NsP1 is the membrane anchor for the complex, forming dodecameric pores that associate monotopically with the membrane in the necks of the spherules to gate their entrance. Enzymatically, nsP1 also has a role in addition of cap0 structures to the 5′ end of the positive-sense viral RNAs. NsP1 possesses both N′7 methyltransferase and guanylyltransferase activity and reverses the order of these reactions. Each nsP1 protomer is built around a methyltransferase fold common to SAM-dependent methyltransferases with additional insertions (membrane binding and oligomerisation (MBO) loops 1 and 2) and extensions (ring aperture membrane binding oligomerisation (RAMBO) domain) that contribute to pore formation, oligomerization, and membrane binding.

The GTP pocket in the capping domain of nsP1 is defined by the tip of strand β4, loop β4-αD, and helix αZ, where loops αC-β4 and β4-αD communicate with the adjacent SAM site. The guanosine base fits in a hydrophobic pocket defined by residues D152, Y248, F241 (β10-11 lid), Y154 (β4-αD loop), and F178 (β5). Base stacking occurs in between D152 and Y248, where the latter residue changes rotamer relative to the SAM-bound and apo structures to become planar with the guanosine. E250 of strand β11 forms H-bonds to the N1 and N2 of the guanosine base, and the carboxylate group of residue D152 (β4-αD loop) maintains a network of H-bonds with GTP-O6 and N7 through an intermediate water molecule. However, relative to other N7 MTases, the GTP pocket is deeper in nsP1, and the guanosine base and ribose are bound further in the fold. The overall effect of this deeper binding pose compared to canonical N7 MTases is to align the alpha phosphate of the GTP with H37, a catalytic residue identified to form a phosphoramide bond in the m7GMP–nsP1 covalent intermediate. Nonetheless, the position of the GTP alpha phosphate is still at 4.8 Å from the histidine side chain Nε and thus too distant to undergo nucleophilic attack. However, as for the SAM ligand, only the base and ribose of the GTP are clearly defined in the maps, suggesting that the phosphates are flexibly bound. The side chains of the positively charged arginine residues lining the path for the phosphates (R92, R70 and R41) are also disordered, with the exception of R41, which becomes ordered relative to the apo and SAM-bound structures and forms H-bonds to the poorly defined β and γ phosphates. In conclusion, the structure clearly shows that many of the residues essential for GTase transfer (see next section) are flexible with only GTP bound, and that further stabilization of the GTP by ligand binding in the SAM site is required for subsequent methyl transfer and GTase reactions.

>[12x]MDPVYVDIDADSAFLKALQRAYPMFEVEPRQVTPNDHANARAFSHLAIKLIEQEIDPDSTILDIGSAPARRMMSDRKYHCVCPMRSAEDPERLANYARKLASAAGKVLDRNISGKIGDLQAVMAVPDTETPTFCLHTDVSCRQRADVAIYQDVYAVHAPTSLYHQAIKGVRLAYWVGFDTTPFMYNAMAGAYPSYSTNWADEQVLKAKNIGLCSTDLTEGRRGKLSIMRGKKLEPCDRVLFSVGSTLYPESRKLLKSWHLPSVFHLKGKLSFTCRCDTVVSCEGYVVKRITMSPGLYGKTTGYAVTHHADGFLMCKTTDTVDGERVSFSVCTYVPATICDQMTGILATEVTPEDAQKLLVGLNQRIVVNGRTQRNTNTMKNYMIPVVAQAFSKWAKECRKDMEDEKLLGVRERTLTCCCLWAFKKQKTHTVYKRPDTQSIQKVQAEFDSFVVPSLWSSGLSIPLRTRIKWLLSKVPKTDLTPYSGDAQEARDAEKEAEEEREAELTLEALPPLQAAQEDVQVEIDVEQLEDRAGAAAHHHHHH>[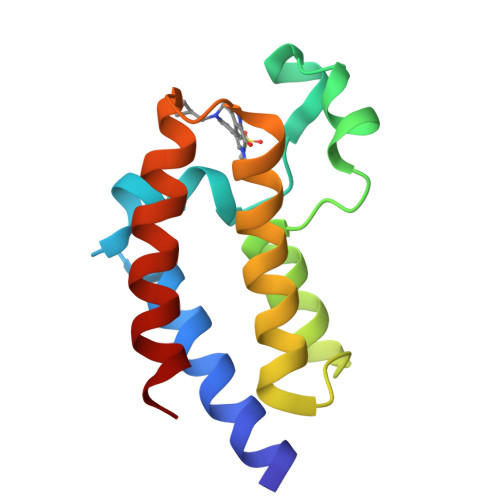2x]SHMEQLKCCSGILKEMFAKKHAAYAWPFYKPVDVEALGLHDYCDIIKHPMDMSTIKSKLEAREYRDAQEFGADVRLMFSNCYKYNPPDHEVVAMARKLQDVFEMRFAKM>[2x]GSHMDSTTIQQNKDTLSQIVVFPTGNYDKNEANAMVNRLANIDGKYLNALKQNNLKIKLLSGKLTDEKEYAYLKGVVPKGWEGTGKTWDDVPGLGGSTV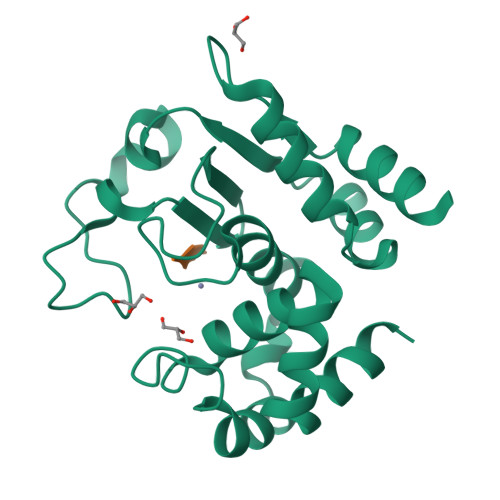ALRIGFSNKGKGHDAINLELHATAHAIDHIVLNDISKSAQFKQIFAKEGRSLGNVNYLGVYPEEFFAESFAYYYLNQDTNSKLKSACPQTYSFLQNLAK;>XEVNP[2x]> GMT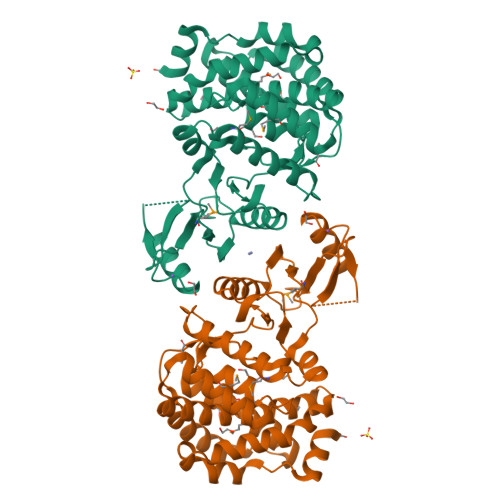SREDEIRDFLATHGYADWNRTPLAGDASSRRYQRLRSPTGAKAVLMDWSPEEGGDTQPFVDLAQYLRNLDISAPEIYAEEHARGLLLIEDLGDALFTEVINNDPAQEMPLYRAAVDLLIHLHDAQTPELARLDPETLSEMTRLAFSEYRYAILGDAAEDNRKRFEHRFAQILSAQLEGDMVFVHRDFHAQNLLWLPEREGLARVGVIDFQDAKLGHRAYDLVSLLQDARRDVPAQVEAQMIDHYIQATGVDESHFRSAYAVIAVQRNMRILGIFARLSQRFGKRHYIEFVPRVWAHFERGLAHPALASAAEEILNALPAPAPEVLERLRA> GSHMKNSVSVDLPGSMKVLVSKSSNADGKYDLIA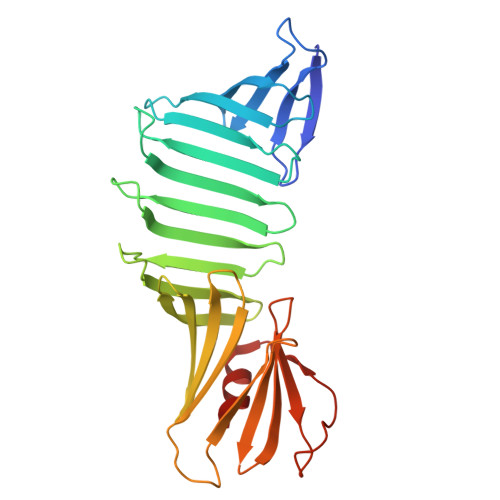TVDALELSGTSDKNNGSGVLEGVKADASKVKLTISDDLGQTTLEVFKSDGSTLVYKYVYSKDKSYTWEYFNEKGEVSYKYIYRADGTRLEYTGIKSDGSGKAKEVLKGYVLEGTLTAEKTTLVVKEGTVTLSKNISKSGEVSVELNDTDSSAATKKTAAWNSGTSTLTITVNSKKTKDLVFTSSNTITVQQYDSNGTSLEGSAVEITKLDEIKNALK>[14x]GAMSGRPLDVLEESLEETVTVRLKDG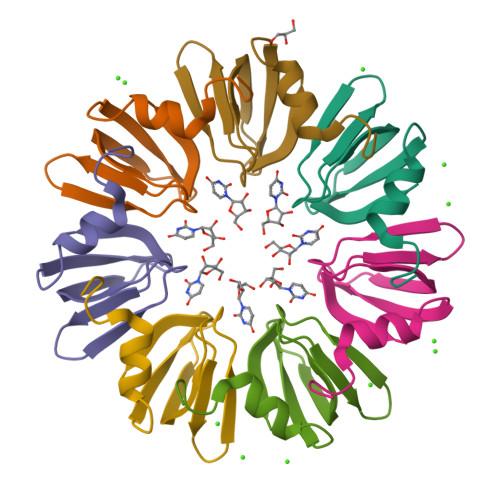DEFTGVLTGYDQHMNVVIEGEDTTIIRGDNVVTIKP>[4x]MGSLPVEGSEEDKSQTGVNRASKGGLIYGNYLHLEKVLNAQELQSETKGNKIHDEHLFIITHQAYELWFKQILWELDSVREIFQNGHVRDERNMLKVVSRMHRVSVILKLLVQQFSILETMTALDFNDFREYLSPASGFQSLQFRLLENKIGVLQNMRVPYNRRHYRDNFKGEENELLLKSEQEKTLLELVEAWLERTPGLEPHGFNFWGKLEKNITRGLEEEFIRIQAKEESEEKEEQV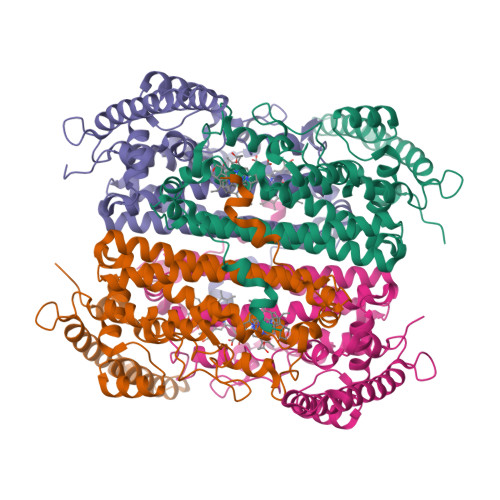AEFQKQKEVLLSLFDEKRHEHLLSKGERRLSYRALQGALMIYFYREEPRFQVPFQLLTSLMDIDSLMTKWRYNHVCMVHRMLGSKAGTGGSSGYHYLRSTVSDRYKVFVDLFNLSTYLIPRHWIPKMNPTIHKFGNSDYKDDDDK>VLFQGPHMLEENIQEKIAFIFNNLSQSNMTQKVEELKETVKEEFMPWVSQYLVMKRVSIEPNFHSLYSNFLDTLKNPEFNKMVLNETYRNIKVLLTSDKAAANFSDRSLLKNLGHWLGMITLAKNKPILHTDLDVKSLLLEAYVKGQQELLYVVP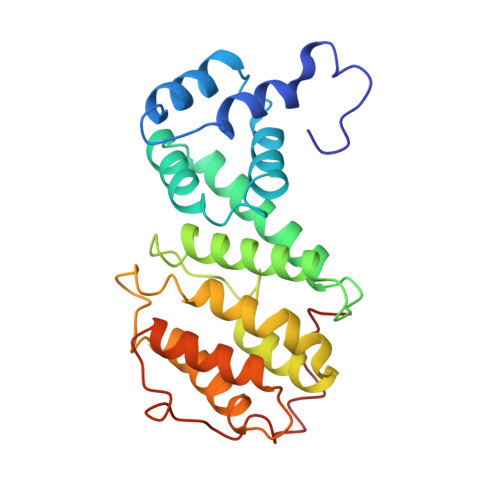FVAKVLESSIRSVVFRPPNPWTMAIMNVLAELHQEHDLKLNLKFEIEVLCKNLALDINELKPGNLLKDKDRLKNLDEQLS[6x]> GPMTTTERPDLAWLDEVTMTQLERNPYEVYERLRAEAPLAFVPVLGSYVASTAEVCREVATSPDFEAVITPAGGRTFGHPAIIGVNGDIHADLRSMVEPALQPAEVDRWIDDLVRPIARRYLERFENDGHAELVAQYCEPVSVRSLGDLLGLQEVDSDKLREWFAKLNRSSTNAAVDENGEFANPEGFAEGDQAKAEIRAVVDPLIDKWIEHPDDSAISHWLHDGMPPGQTRDREYIYPTIYVYLLGAMQEPGHG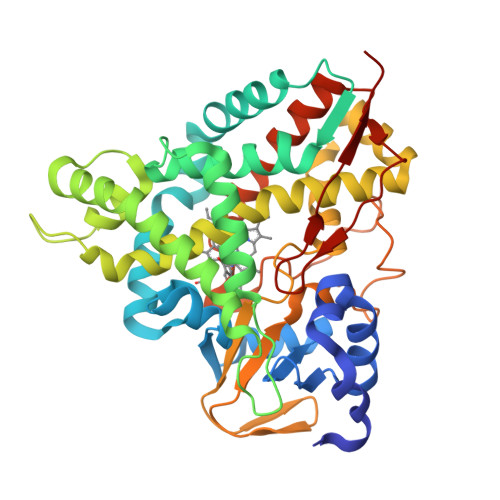MASTLVGLFSRPEQLEEVVDDPTLIPRAIAEGLRWTSPIWSATARISTKPVTIAGVDLPAGTPVMLSYGSANHDTGKYEAPSQYDLHRPPLPHLAFGAGNHACAGIYFANHVMRIALEELFEAIPNLERDTREGVEFWGWGFRGPTSLHVTWEV> GAMAATAAEAVASGSGEPREEAGALGPAWDESQLRSYSFPTRPIPRLSQSDPRAEELIENEEPVVLTDTNLVYPALKWDLEYLQENIGNGDFSVYSASTHKFLYYDEKKMANFQNFKPRSNREEMKFHEFVEKLQDIQQRGGEERLYLQQTLNDTVGRKIVMDFLGFNWNWINKQQGKRGWGQLTSNLLLIGMEGNVTPAHYDEQQNFFAQIKGYKRCILFPPDQFECLYP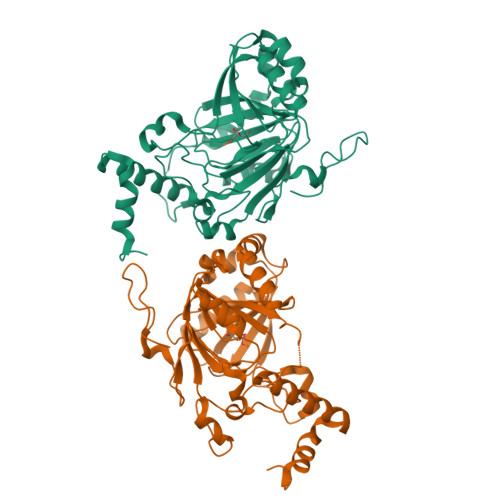YPVHHPCDRQSQVDFDNPDYERFPNFQNVVGYETVVGPGDVLYIPMYWWHHIESLLNGGITITVNFWYKGAPTPKRIEYPLKAHQKVAIMRNIEKMLGEALGNPQEVGPLLNTMIKGRYN> ER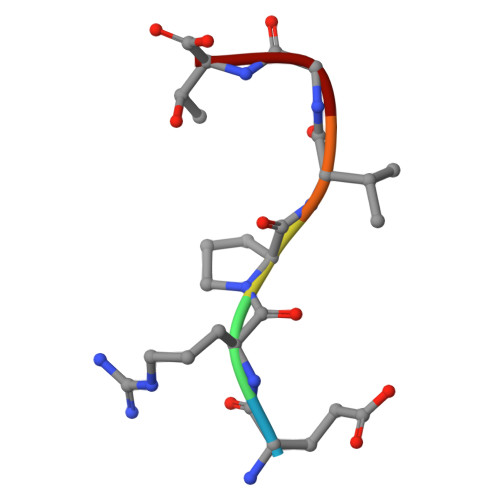PVGT>[2x]SMGGTHIDLLFHPPRAHLLTIKETIRKMIK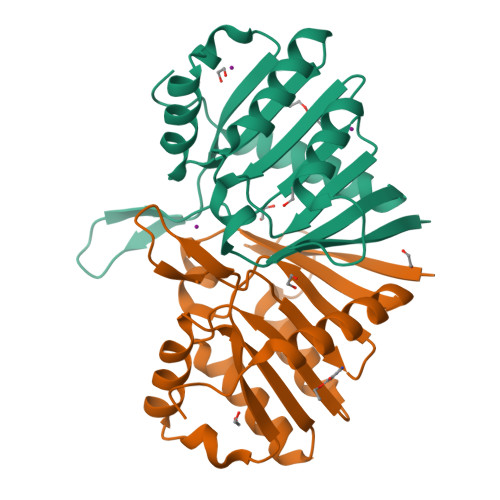EARKVIALVMDIFTDVDIFKEIVEASTRGVSVYILLDESNFNHFLNMTEKQGCSVQRLRNIRVRTVKGQDYLSKTGAKFHGKMEQKFLLVDCQKVMYGSYSYMWSFEKAHLSMVQIITGQLVESFDEEFRTLYARSCVPSSFAQEESARV> MAFNDLLQQVGGVGRFQQIQVTLVVLPLLLMASHNTLQNFTAAIPTHHCRPPADANLSKNGGLEVWLPRDRQGQPESCLRFTSPQWGLPFLNGTEANGTGATEPCTDGWIYDNSTFPSTIVTEWDLVCSHRALRQLAQSLYMVGVLLGAMVFGYLADRLGRRKVLILNYLQTAVSGTCAAFAPNFPIYCAFRLLSGMALAGISLNCMTLNVEWMPIHTRACVGTLIGYVYSLGQFLLAGVAYAVPHW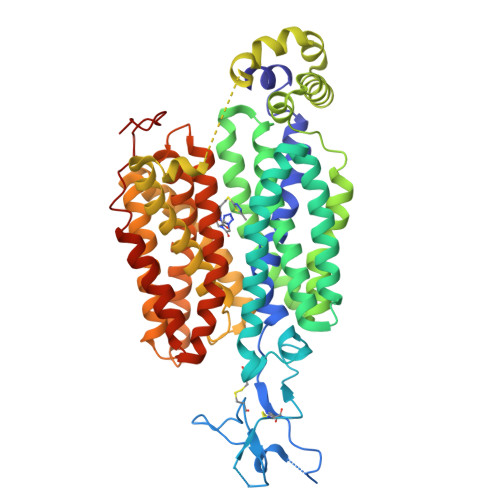RHLQLLVSAPFFAFFIYSWFFIESARWHSSSGRLDLTLRALQRVARINGKREEGAKLSMEVLRASLQKELTMGKGQASAMELLRCPTLRHLFLCLSMLWFATSFAYYGLVMDLQGFGVSIYLIQVIFGAVDLPAKLVGFLVINSLGRRPAQMAALLLAGICILLNGVIPQDQSIVRTSLAVLGKGCLAASFNCIFLYTGELYPTMIRQTGMGMGSTMARVGSIVSPLVSMTAELYPSMPLFIYGAVPVAASAVTVLLPETLGQPLPDTVQDLESR Our results supported a “two-arm” architecture of the STRIPAK complex, with the PP2Aa/c-bound STRNs acting as an organizing center to hold Hippo or other MST kinases with STRIP1 as one arm and SIKE1-SLMAP as the other. Moreover, we determined the crystal structures of the second coiled-coil domain of SIKE1 alone, and in complex with an STRN3 peptide, as well as the structure of the first coiled-coil domain of SIKE1 in complex with the first coiled-coil domain of SLMAP. SIKE1 functions to bridge SLMAP through CC1 on one hand and STRN3 through CC2 on the other. In particular, we discovered SIKE1 as a key adaptor that recruits MST-bound SLMAP to PP2A-bound STRN, forming a molecular arm MST-SLMAP-SIKE1-STRN-PP2Aa/c.

In the structure of the STRN3-SIKE1 CC2 complex, two SIKE1 CC2 molecules (chains A and B) formed a homodimer to bind one STRN3 peptide, resulting in a 2:1 heterotrimer. STRN3 folded as an alpha helix with a C-terminal turn. Many residues mediating homotetramerization of SIKE1 CC2 in the apo state were now found to contact the STRN3 peptide. For example, residues H97, A100, L103, I104, and K107 in chain B, and L101, M105, and Y108 in chain A of SIKE1 CC2 formed a hydrophobic patch with residues L179, Y182, L183, V186, and Y188 of STRN3. In addition, the side chains of residues E96 in chain B and R109 in chain A of SIKE1 CC2 formed two salt bridges and three hydrogen bonds with R176 and E185 of STRN3. Structural comparison revealed significant conformational changes in SIKE1 CC2 upon STRN3 binding. Secondly, in the presence of STRN3, SIKE1 CC2 became an asymmetric homodimer (chains A and B) with C-terminal regions in both chains bending closer to each other (about 22°). The bended chain B occupied a position corresponding to chain A′ of SIKE1 CC2 in the apo state. Since the STRN3 bound to SIKE1 as if it were a helical chain of SIKE1, the bending of SIKE1 CC2 thus blocked the binding of another STRN3 peptide, explaining the 2:1 stoichiometry. Structure-guided mutational analysis showed that mutations of STRN3 (R176A/E185A and L179D/V186D) or SIKE1 (E96A/R109A and A100D/M105E) on the SIKE1-STRN3 interface disrupted the complex formation.

>STMALLSQENTQIRDLQQENRELWISLEEHQDALELIMSKYRKQMLQLMVAKKA[2x];> PQNSQLTWKQGRQLLRQYLQEVGYTD>AAPLPELLSNNGKHALMVDGAPYIILGSQTNNSSNYPDALKDVWPSMEKMGANTLSIPVAWEQIEPVEGQFDFSFVDVLLKEARQRKVRLVLLWFATWKNNAPHYAPAWVKLDNARFPRVVKEDGDTLNSLSPLGQNTLAADKKAFVELMKYLAKRDKDHTVIMVQVQNEVGTYGAVRDYSPMAQAVFNAAVPDDLIQKLQLKPGTWSQVFGRDADEFFHAYQIARYCDEVTVAGKAIKNLPMYVNVALRNPFNPGLPGQYSSGGGTDNVLHIWKAAAPNIDLIAPDIYFRDYKTVSKVLELYTRPDNALFVAEIGNDQPFARYLFPTLGKGGIGFSPFGMDDTDYTNYPLGAKVYNDETIEQFAQVYRLVNPMMREWARLSYQGQVWGVAEPLDSTTETQKIWNAEATPEEKEQHKKDRASALTQQLDLGLWDAEVTYGRPMFWVTPPEGNTPAAGGALIAQLDDNEYLVTAYKARVEFKPSQELAGKKFMIERVEEGRFEKGKWVMERVWNGDQTDWGLNFTDRPHLLRVKMASYSVQ[8x]

Genome walking in silico revealed the presence of open reading frames encoding a predicted β-galactosidase from glycoside hydrolase (GH) family 35 (CjBgl35A, encoded by locus tag CJA_2707, bgl35A), a predicted TonB-dependent receptor (TBDR, encoded by CJA_2709), and a predicted α-l-fucosidase from glycoside hydrolase family 95 (CjAfc95A, encoded by CJA_2710, afc95A) upstream from the gene encoding the known α-xylosidase CjXyl31A (CJA_2706, xyl31A). The data indicate that CjBgl35A acts strictly as an exo-galactosidase that requires terminal galactosyl moieties on XyGOs. Rather, the specificity of CjBgl35A is similar to plant β-galactosidases with a general ability to remove side-chain galactosyl units from xyloglucan polysaccharides; the GH35 member from A. thaliana, Bgal10 (At5g63810) produces XXLG and XXXG sequentially due to a preference for the underlined side-chain in XLLG (Sampedro et al., 2012 and references therein). The liberated XyGOs are then imported into the periplasm via the TBDR, where the exo-glycosidases CjXyl31A, CjBgl35A, and CjAfc95A work in concert, together with a currently unidentified β-glucosidase(s), to yield monosaccharides for further catabolism.

Given its poor sequence similarity to other GH35 enzymes (vide supra), this two-domain fold exhibits low homology to other currently known protein structures; only one significant structural match to another bacterial GH35 β-galactosidase, from Caulobacter crescentus strain CB15, was found. The (β/α)8 structure of the CjBgl35A N-terminal catalytic domain reveals a centrally positioned cleft running laterally across the open end of the barrel. This topology appears to be consistent with the requirement for binding of extended, branched oligo/polysaccharide substrates such as XyGOs and/or XyG and thus the cleft was anticipated to contain the catalytic active site. Despite the observation of separate protein domains, it seems likely that these together solely constitute a catalytic module, i.e. a distinct biochemical/biological function is not indicated. Structure/sequence homology searching of the C-terminal region in isolation produced no significant results that would indicate similarity to known regulatory or carbohydrate-binding modules (CBMs), despite the observation of a trough-like surface somewhat reminiscent of a substrate recognition cleft. In addition, the observation that the early part of the C-terminal domain is formed from a distortion of the final helix of the barrel domain, and that the initial β-strand of this domain stacks directly against the penultimate barrel helix, strongly suggests a rigid, monolithic structure.>GCEASAFIVNGDKEELFLERVDKLIPTEEGLLLENIFGQRKVIKAKIKRLELVDHRILLERED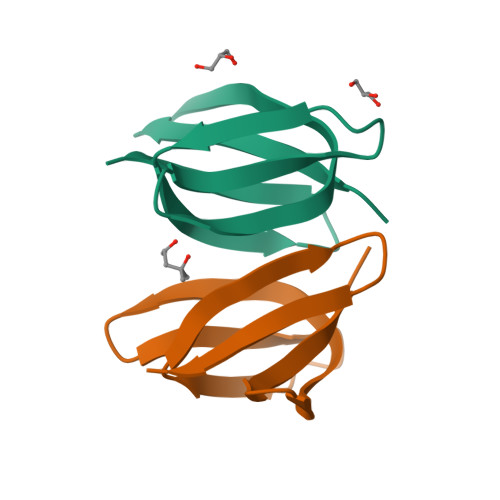[6x]8-methoxy-2,3-dimethylquinoxalin-5-ol | C11 H12 N2 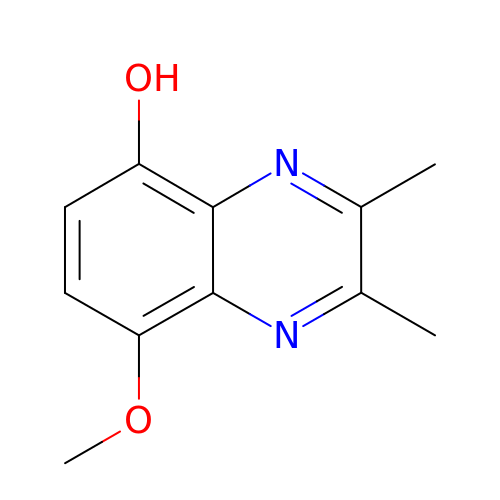O2 | YKNPPZPHWDKZHL-UHFFFAOYSA-N> IVGGRRARPHAWPFMVSLQLRGGHFCGATLIAPNFVMSAAHCVANVNVRAVRVVLGAHNLSRREPTRQVFAVQRIFENGYDPVNLLNDIVILQLNGSATINANVQVAQLPAQGRRLGNGVQCLAMGWGLLGRNRGIASVLQELNVTVVTSLCRRSNVCTLVRGRQAGVC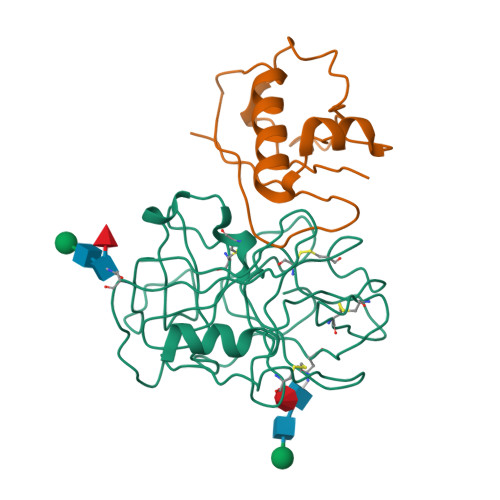FGDSGSPLVCNGLIHGIASFVRGGCASGLYPDAFAPVAQFVNWIDSIIQ;> GSTDSNNGYKELTMDGKHTVPYTISVDGITALHRTYFVFPENKKVLYQEIDSKVKNELASQRGVTTEKINNAQTATYTLTLNDGNKKVVNLKKNDDAKNSIDPSTIKQIQIVVK> MGGEIITLQAGQCGNHVGKFLWSQLAKEHAIGTDGLSQLPDSSTERDDDTKPFFRENSRNKFTPRAIMMDSEPSVIADVENTFRGFFDPRNTWVASDGASAGNSWANGYDIGTRNQDDILNKIDKEIDSTDNFEGFQLLHSVAGGTGSGLGSNLLEALCDRYPKKILTTYSVFPARSSEVVVQSYNTILALRRLIEDSDATVVFDNASLLNISGKVFRNPNIDLQHTNQLISTIISSVTNSIRFPSYMYSSMSSIYSTLIPSPELHFLSPSFTPFTSDYIHDDIAHKGHSSYDVMLDLLDPSNSLVSTAMNNPTYFNVYNTIIGNVEPRQISRAMTKLQQRIKFPSWSSSAMHVNIGRRSPYLPLQPNENEVSGMML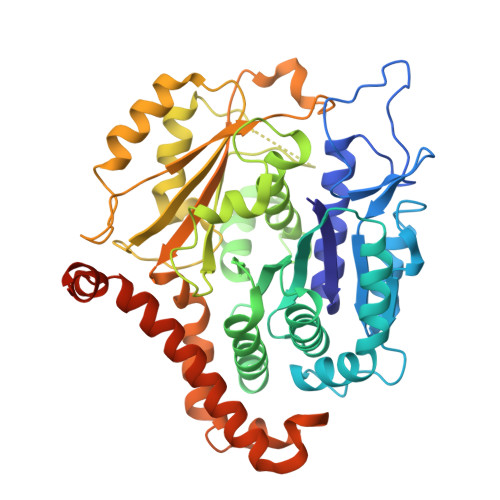SNMSTVVNVFENACNTFDKVFAKGAFLNNYNVGDLFQSMQNVQDEFAESREVVQSLMEDYVAAEQDSYLDDVLVDDENMVGELEEDLDADGDHKLV>GHMDSTTIQQNKDTLSQIVVFPTGNYDKNEANAMVNRLANIDGKYLNALKQNNLKIKLLSGKLTDEKEYAYLKGVVPKGWEGTGKTWDDVPGLGGSTVALRIGFSNKGKGHDAINLELHATAHAIDHIVLNDISKSAQFKQIFAKEGRSLGNVNFLGVYPEE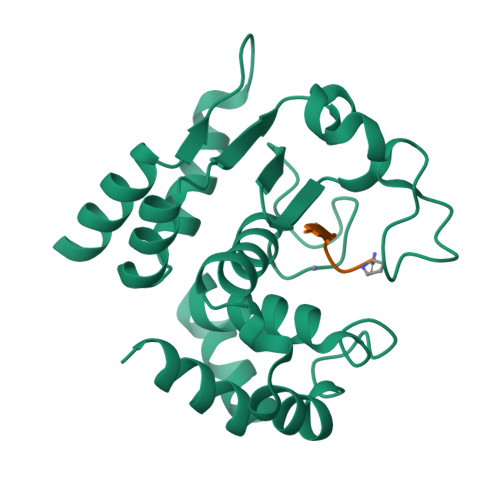FFAESFAYYYLNQDTNSKLKSACPQTYSFLQNLAK[2x];>XEVAPPVP[2x]> MAKDIEISASESKFILEALRQNYRLDGRSFDQFRDVEITFGKEFGDVSVKMGNTKVHCRISCQIAQPYEDRPFEGLFVISTEISPMAGSQFENGNITGEDEVLCSRIIEKSVRRSGALDVEGLCIVAGSKCWAVRADVHFLDCDGGFIDASCIAVMAGLMHFKKPDITVHGEQIIVHPVNEREPVPLGILHIPICVTFSFFNPQDTEENIKGETNSEISIIDATLKEELLRDGVLTVTLNKNREVVQVSKAGGLPMDALTLMKCCHEAYSIIEKITDQILQLLKEDSEKRNKYAAMLTSENAREI;> MSRLEIYSPEGLRLDGRRWNELRRFESSINTHPHAADGSSYMEQGNNKIITLVKGPKEPRLKSQMDTSKALLNVSVNINKFSKFERSKSSHKNERRVLEIQTSLVRMFEKNVMLNIYPRTVIDIEIHVLEQDGGIMGSLINGITLALIDAGISMFDYISGISVGLYDTTPLLDTNSLEENAMSTVTLGVVGKSEKLSLLLVEDKIPLDRLENVLAIGIAGAHRVRDLMDEELRKHAQKRVSNASAR;> VRSRNGGATKIVREHYLRSDIPCLSRSCTKCPQIVVPDAQNELPKFILSDSPLELSAPIGKHYVVLDTNVVLQAIDLLENPNCFFDVIVPQIVLDEVRNKSYPVYTRLRTLCRDSDDHKRFIVFHNEFSEHTFVERLPNETINDRNDRAIRKTCQWYSEHLKPYDINVVLVTNDRLNREAATKEVESNIITKSLVQYIELLPNADDIRDSIPQMDSFDKDLERDTFSDFTFPEYYSTARVMGGLKNGVLYQGNIQISEYNFLEGSVSLPRFSKPVLIVGQKNLNRAFNGDQVIVELLPQSEWKAPSSIVLDSEHFDVNDNPDIEAGDDDDNNESSSNTTVISDKQRRLLAKDAMIAQRSKKIQPTAKVVYIQRRSWRQYVGQLAPSSVDPQSSSTQNVFVILMDKCLPKVRIRTRRAAELLDKRIVISIDSWPTTHKYPLGHFVRDLGTIESAQAETEALLLEHDVEYRPFSKKVLECLPAEGHDWKAPTKLDDPEAVSKDPLLTKRKDLRDKLICSIDPPGCVDINDALHAKKLPNGNWEVGVHIADVTHFVKPGTALDAEGAARGTSVYLVDKRIDMLPMLLGTDLCSLKPYVDRFAFSVIWELDDSANIVNVNFMKSVIRSREAFSYEQAQLRIDDKTQNDELTMGMRALLKLSVKLKQKRLEAGALNLASPEVKVHMDSETSDPNEVEIKKLLATNSLVEEFMLLANISVARKI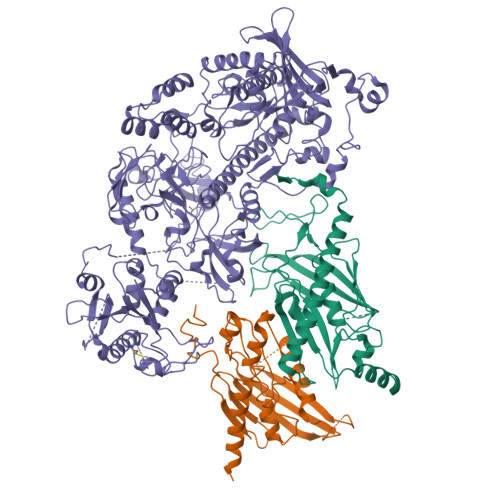YDAFPQTAMLRRHAAPPSTNFEILNEMLNTRKNMSISLESSKALADSLDRCVDPEDPYFNTLVRIMSTRCMMAAQYFYSGAYSYPDFRHYGLAVDIYTHFTSPIRRYCDVVAHRQLAGAIGYEPLSLTHRDKNKMDMICRNINRKHRNAQFAGRASIEYYVGQVMRNNESTETGYVIKVFNNGIVVLVPKFGVEGLIRLDNLTEDPNSAAFDEVEYKLTFVPTNSDKPRDVYVFDKVEVQVRSVMDPITSKRKAELLLK> MGFLDGKRILLTGLLSNRSIAYGIAKACKREGAELAFTYVGDRFKDRITEFAAEFGSELVFPCDVADDAQIDALFASLKTHWDSLDGLVHSIGFAPREAIAGDFLDGLTRENFRIAHDISAYSFPALAKAALPMLSDDASLLTLSYLGAERAIPNYNTMGLAKAALEASVRYLAVSLGAKGVRVNAISAGPIKTLAASGIKSFGKILDFVESNSPLKRNVTIEQVGNAGAFLLSDLASGVTAEVMHV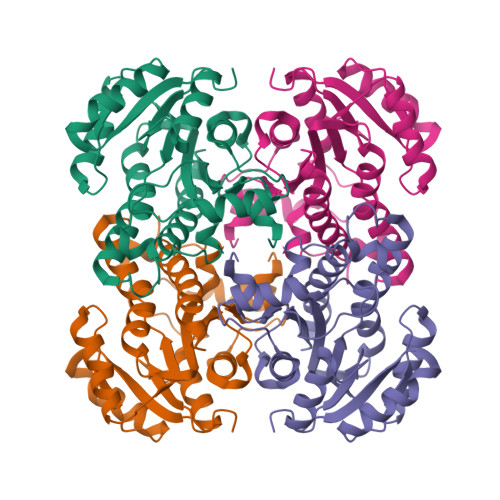DSGFNAVVGGMAGLEEKLAAALEHHHHHH> TRKYLNTNVTPHLLAGMRLIAVQQPEDPLRVLGEYLIE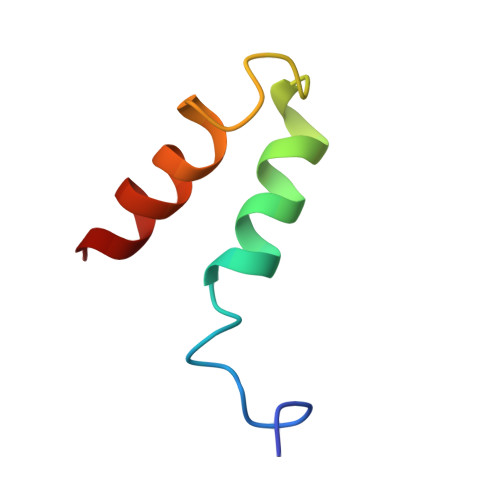QSNI> YSAM;> AKCVSYGVAQIKAPALHSQGYTGSNVKVAILDTGIDSSHPDLNVAGGASFVPSETNPFQDNSSGGTHIAGTVLAVAPSASLYAVKVLGADGKGQASWIINGIEWAIANNMDVINMSLGSPSGSAAVKAAVDKAVASGVVVVAAAGNSGTSGSSSTVTYPAKYPSVIAVGAVDSSNQRAPFSSVGPELDVM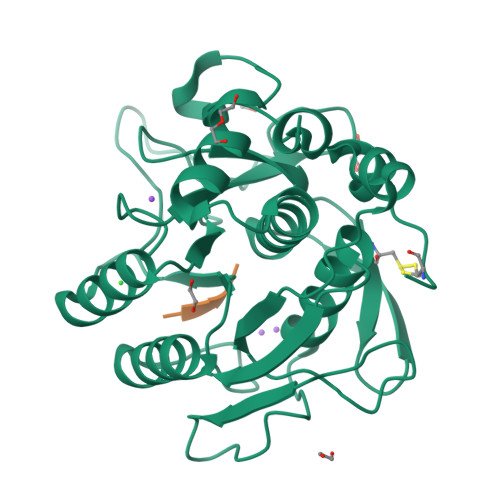APGVSICSTLPGGKYGALSGTSMASPHVAGAAALILSKHPNWTNTQVRSSLENTATKLGDSFYYGKGLINVEAAAQ>[2x]GSHMPTRKKFVAGNWKMNTTLAEAKALGAAVAKGVTDDRVTVAVFPPYPWLTAVGEVLKGSPVALGAQDVSSEKKGAFTGEVSPAMLLETGCKYALIGHSERRHIIGESETFINHKVHTALEEGLSVVLCMGETLAERERGLQERVFQRQVYAACAGLTDEQFGRIVIAYEPVWAIGTGKVATPEQAQEAH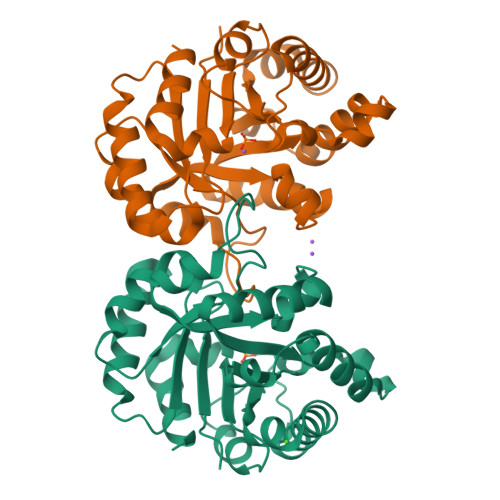AFVRSKLRLLYGDKIADSTPIVYGGSVTPDNTVGLMSQPDVDGALVGGASLKADSFLAIVKAAG> GPAGQFIRDTAPDGRVYKLYIPSGYNGSTPLPLVVMLHGCTQNPDDFAAGTEMNVYAEQNNFLVAYPEQPSSANLNKCWNWFDSNHQSRGRGEPASIAGVVEDVKRNYSVDSRRVYAAGLSAGGAMSVIMGATYPDVFAAIGVGSGLEYKAATSMTSAYMAMINGGPDPVQQGNLAYQAMGSHARVVPVIVFHGTSDYTVYPVNGHQVISQWAQTNDRAGDGVDNNHIDDQADVTMNGSVPNGRTYTRYLYKDQNGNVVMEKIMVNGMGHAWSGGSTAGTYTDPAGPEASSMMWSFFVNHPK

Recently, a promiscuous PHBase from the thermophilic soil bacterium Lihuaxuella thermophila (LtPHBase) was identified. LtPHBase can accommodate many substrates, including PHB granules and films and PHB block copolymers, as well as the unrelated polymers polylactic acid (PLA) and polycaprolactone (PCL). LtPHBase belongs to the secreted subfamily of PHBases, which most likely function to scavenge hydroxybutyrate (HB) from a few environmental biopolyester polymers.

To test the hypothesis that LtPHBase might adopt different active-site loop conformations in the absence of bound ligands, we identified new crystallization conditions that do not include IPA and we used PEG 400 as the cryoprotectant instead of EG. The overall root-mean-squared deviation (r.m.s.d.) is 0.2 Å, indicating a high level of agreement between the two structures. The two most notable differences are distal from the active site. Firstly, the loop comprising residues 221–225 is disordered in apo LtPHBase, whereas in the IPA/EG-bound structure the loop was readily modeled. Secondly, the five N-terminal residues adopt different conformations. These changes in the structure can be attributed to differences in crystal contacts and suggest flexibility in these regions. Slight changes in the surface helix (residues 155–164) appear to be primarily responsible for this difference. Most notably, in the apo structure Met155 is oriented towards Phe81 and away from the Tyr159 side chain, which itself is in a new orientation compared with IPA/EG-bound LtPHBase. LtPHBase is likely to prefer lower-molecular-mass, non-film polymers due to the apparent lack of conformational access to the catalytic triad, as seen in our apo structure.> LGSGCHHRICHCSNRVFLCQESKVTEIPSDLPRNAIELRFVLTKLRVIQKGAFSGFGDLEKIEISQNDVLEVIEADVFSNLPKLHEIRIEKANNLLYINPEAFQNLPNLQYLLISNTGIKHLPDVHKIHSLQKVLLDIQDNINIHTIERNSFVGLSFESVILWLNKNGIQEIHNCAFNGTQLDELNLSDNNNLEELPNDVFHGASGPVILDISRTRIHSLPSYGLENLKKLRARSTYNLKKLPTLEKLVALMEASLTYPSHCCAFANWRRQISELHPICNKSILRQEVDYMTQARGQRSSLAEDNESSYSRGFDMTYTEFDYDLCNEVVDVTCSPKPDAFNPCEDIMGYNILRVLIWFISILAITGNIIVLVILTTSQYKLTVPRFLMCNLAFADLCIGIYLLLIASVDIHTKSQYHNYAIDWQTGAGCDAAGFFTVFASELSVYTLTAITLERWHTITHAMQLDCKVQLRHAASVMVMGWIFAFAAALFPIFGISSYMKVSICLPMDIDSPLSQLYVMSLLVLNVLAFVVICGCYIHIYLTVRNPNIVSSSSDTRIAKRMAMLIFTDFLCMAPISFFAISASLKVPLITVSKAKILLVLFHPINSCANPFLYAIFTKNFRRDFFILLSKCGCYEMQAQIYRTETSSTVHNTHPRNGHCSSAPRVTNGSTYILVPLSHLAQN

Follicle stimulating hormone (FSH) is an essential glycoprotein hormone for human reproduction, which functions are mediated by a G protein-coupled receptor, FSHR. There are three members of glycoprotein hormone receptors, FSHR, LHCGR and TSHR, which are activated to mainly couple the Gs protein and lead to up-regulation of the secondary message cAMP in cells. FSH acts through FSHR, which is mainly expressed in gonads (ovaries in female and testes in male). Here we report cryo-EM structures of FSHR in both inactive and active states, with the active structure bound to FSH and an allosteric agonist compound 21 f.

To obtain stable inactive FSHR proteins for cryo-EM structure determination, a small molecular antagonist, compound 2427, was added during FSHR expression and purification. Through numerous data collection, we were able to obtain a structure of wild type FSHR in the inactive state at a global resolution of 6.01 Å. The EM map was sufficient to place the receptor ECD and TMD, while the density of compound 24 was not observed. Due to the relatively low resolution of the inactive FSHR map, we only built a poly-alanine model for the inactive FSHR structure. In the inactive FSHR structure, the ECD conformation is closely titled toward the membrane layer and the TMD conformation is very similar to the inactive β2AR31. Structural comparison of the inactive FSHR with the inactive LHCGR and TSHR structures reveals that all three receptors have a similar ECD down conformation. The ECD of FSHR has a nearly identical position as the LHCGR ECD but a 7°–8° rotation close to the membrane layer relative to the ECD of the inactive TSHR. Interestingly, the hinge helix in the inactive FSHR structure is elongated and shows different orientation from the hinge helix in the active FSHR structure, highlighting that hinge helix plays an important role during FSHR activation. In contrast, the hinge helix in the inactive FSHR structure shows rare interactions with ECL1 by rotating approximately 30° counter-clockwise relative to the hinge helix from the active FSHR structure, thus confirming that the interactions between hinge helix and ECL1 is critical for FSHR activation.> KETKNVPFKLKNAAPVIFSHDIHLKKYNNNCRICHIALFDLRKPKRYTMLDMEKGKSCGACHTGMK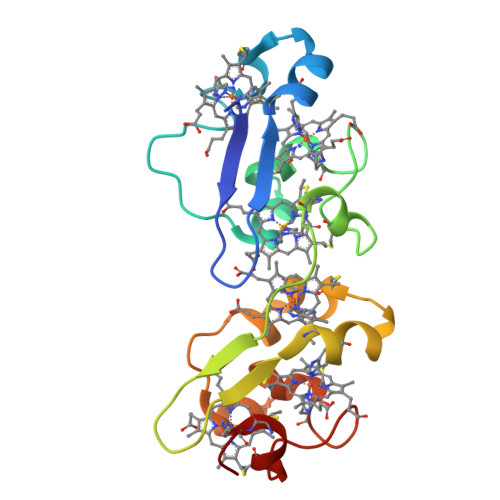AFSVADDSQCVRCHSGSARPVAYRMKGAGEAVFSHEVHVPMLEGKCRTCHSNREITGGRNVTMAQMEKGKSCGACHNDKMAFTVAGNCGKCHKGM> MQDNSRYTHFLTQHYDAKPQGRDDRYCESIMRRRGLTSDRCKPINTFIHGNKRSIKAICENKNGNPHRENLRISKSSFQVTTCKLHGGSPWPPCQYRATAGFRNVVVAC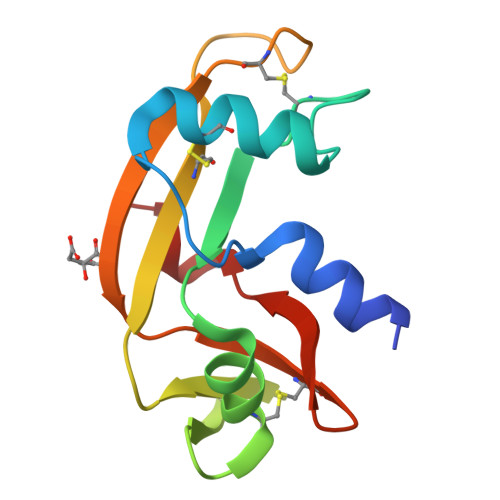ENGLPVHLDQSIFRRP> ASLCLSQQFKAQGDYILGGLFPLGSTEEATLNQRTQPNSIPCNRFSPLGLFLAMAMKMAVEEINNGSALLPGLRLGYDLFDTCSEPVVTMKSSLMFLAKVGSQSIAAYCNYTQYQPRVLAVIGPHSSELALITGKFFSFFLMPQVSYSASMDRLSDRETFPSFFRTVPSDRVQLQAVVTLLQNFSWNWVAALGSDDDYGREGLSIFSSLANARGICIAHEGLVPQHDTSGQQLGKVLDVLRQVNQSKVQVVVLFA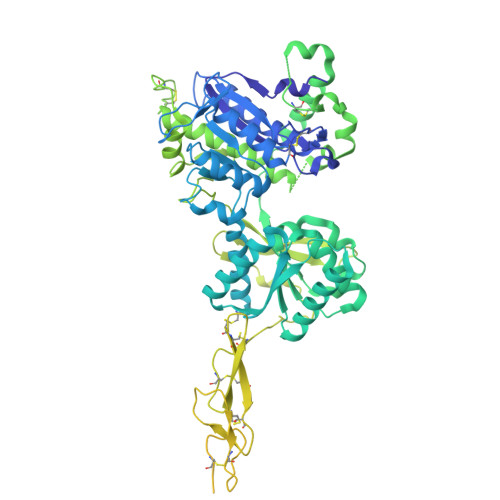SARAVYSLFSYSIHHGLSPKVWVASESWLTSDLVMTLPNIARVGTVLGFLQRGALLPEFSHYVETHLALAADPAFCASLNAELDLEEHVMGQRCPRCDDIMLQNLSSGLLQNLSAGQLHHQIFATYAAVYSVAQALHNTLQCNVSHCHVSEHVLPWQLLENMYNMSFHARDLTLQFDAEGNVDMEYDLKMWVWQSPTPVLHTVGTFNGTLQLQQSKMYWPGNQVPVSQCSRQCKDGQVRRVKGFHSCCYDCVDCKAGSYRKHPDDFTCTPCNQDQWSPEKSTACLPRRPKFLAWGEPVVLSLLLLLCLVLGLALAALGLSVHHWDSPLVQASGGSQFCFGLICLGLFCLSVLLFPGRPSSASCLAQQPMAHLPLTGCLSTLFLQAAETFVESELPLSWANWLCSYLRGLWAWLVVLLATFVEAALCAWYLIAFPPEVVTDWSVLPTEVLEHCHVRSWVSLGLVHITNAMLAFLCFLGTFLVQSQPGRYNRARGLTFAMLAYFITWVSFVPLLANVQVAYQPAVQMGAILVCALGILVTFHLPKCYVLLWLPKLNTQEFFLGRNAKKAADENSGGGEAAQGHNE>[2x]GPLGSMITRNPIVPENHVSNPVTDYEFNQDQSCLILSTLKSFEIYNVHPVAHIMSQEMRHLSKVRMLHRTNYVAFVTGVKEVVHIWDDVKKQDVSRIKVDAPVKDLFLSREFIVVSYGDVISVFKFGNPWKRITDDIRFGGVCEFSNGLLVYSNEFNLGQIHITKLQSSGSATTQDQGVQQKAILGKGVLIKAHTNPIKMVRLNRKSDMVATCSQDGTII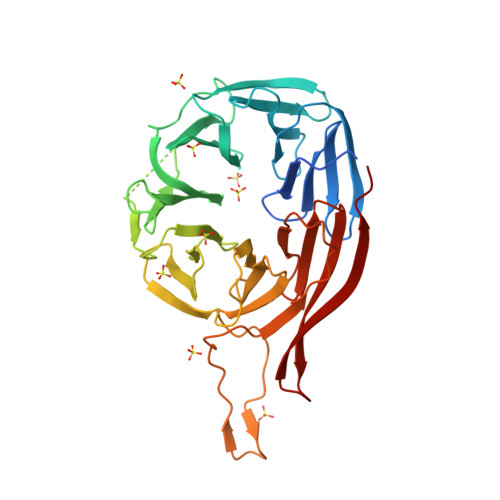RVFKTEDGVLVREFRRGLDRADVVDMKWSTDGSKLAVVSDKWTLHVFEIFNDQDNKRHALKGWINMKYFQSEWSLCNFKLSVDKHVRGCKIAWISESSLVVVWPHTRMIETFKVVFDDEMERWLIQMDQREQLMI> MASWSHPQFEKGAENLYFQSNAMKLAQGAFVDVIRIGALSPPTDQRSLWARTLLSEAVDQGLDSLPVPLQDVSTFTVTLQPALAVRLKALADQHNTPVSVYAAGLIEAMRRRSESGSVAEAPMELPADALPGEGAVREVLRPLLKQAAEKTAAGKIVFAEAATGTGKGRMIASLAAAAAIKGDTVVVSAPLAVTWQLVNDMKDIPEVRRVGLTLSLGRPNFISPQRTLEWAIDNERADLAAWIEGGGKPLSLRSMETSKVISHELCWLLEDALLLAEDLPADSLLLTSEDPADCPAQQLYVAMRSNYTEAGIILCSHFMLAAHTRMMQMRGLGNDEELDDEAPTGLSLPHFIDTLIVDEAHLLEQAFASVYTHTLRLRPLMRTIEGLGSRGRKPALDALKELFTQMQVASARSTNTSLNVPLSDVPELIPALKDTVKTLGALPTKGMSRDARSVIRIATRAANDALSGHSRLRIEVTPVHSYPMLLSGRSNLQRALLGLWNATGGATLVSATLFTTGDNGSLTRWKLEVPTERAAFLPPVHPAWTTAPVLLHKEFCAHEPDDSPEWATECAQTIQGVASTAQGGTLVLCTSYQNTELLAGRLGAALGDRLIVQSKTSSAATCLAQFKAKHKAGIRPVWLGLGAAWTGIDLSDHSLPDNPELDRLLSDLVITRIPVGQNRSLTHERRTAIGGFRIISQEAAWHFRQGLGRLVRRPGVTHKNLWVLDARIYGGAAWVAPFRQILDRYKKA

CRISPR-associated DinG protein (CasDinG) is essential to type IV-A CRISPR function. Here, we demonstrate that CasDinG from Pseudomonas aeruginosa strain 83 is an ATP-dependent 5′-3′ DNA translocase that unwinds double-stranded (ds)DNA and RNA/DNA hybrids. The crystal structure of CasDinG reveals a superfamily 2 helicase core of two RecA-like domains with three accessory domains (N-terminal, arch, and vestigial FeS). CasDinG is an essential component of the type IV-A CRISPR Cas system, which clears bacteria of invasive nucleic acid and silences gene expression.

To better understand the function of the accessory domains we determined the crystal structure of CasDinG from P. aeruginosa strain 83 at 2.95 Å resolution with an Rwork/Rfree of (18.5 / 21.5) in space group P 65. We solved the structure by molecular replacement using an AlphaFold2 model of N-terminally truncated CasDinG. The CasDinG structure reveals a SF2 helicase core of two RecA-like helicase domains (HD1 and HD2) and two accessory domains inserted within HD1 (vFe/S and arch domain). An N-terminal domain of 103 amino acids was not observed in the electron density. The alignment revealed that the HD domains of CasDinG are in a wider, or ‘extra open’, conformation than the HD domains of the binary E. coli DinG structure. The extra open conformation may be a crystallographic artifact, or the result of having no ssDNA bound in the CasDinG structure. The first insert (residues 195–275) consists of a four alpha-helix bundle that aligns with the E. coli DinG FeS cluster domain with an RMSD of 2.3 Å using the Coot Secondary Structure Matching tool. Despite this conserved topology, CasDinG lacks three of the four cysteines observed in E. coli DinG that coordinate the FeS cluster, and no FeS cluster is observed in the electron density of the CasDinG structure. In CasDinG, the lack of a stabilizing FeS cluster is compensated for by a salt bridge formed between residues R204 and D269. Notably, analysis of CasDinG crystal packing suggests that the vFeS position that sterically blocks ssDNA binding is likely a crystallographic artifact, indicating a conformational rearrangement of the domain that allows for ssDNA would likely be allowed in solution.AaRSs catalyze the attachment of the correct amino acid to its cognate tRNA which then is used in protein synthesis on ribosomes. Phylogenetically phenylalanyl-tRNA synthetase (PheRS), belongs to the class II aaRSs, and it is a dimer of heterodimers (αβ)2, containing two α- (PheS) and two β- (PheT) subunits. Structural studies of PheRS have shown that the α subunit binds L-Phe and ATP and is responsible for esterification catalysis. At the same time, the β subunit is involved in the recognition of the cognate tRNA molecule and editing of mis-charged tRNA.

The protein-fragment interactions were analyzed using crystal structures for five of those fragments complexed with MtPheRS/tRNAPhe (DDD00107555 (D-555), DDD01008876 (D-876), DDD00805735 (D-735), DDD00079004 (D-004) and DDD00067116 (D-116)). The FMO analysis indicates that the sulphonamide group of the D-735 interacts with αArg201 and αGln158 through strong hydrogen bonds. Also, the aniline nitrogen form hydrogen bond with the αGlu217 of D-735 fragment. Synthesis of L-Phe-AMP was inhibited the least by D-735 fragment. In the present study, the 3’ CCA tail of the tRNAPhe in the αβ heterodimer bound to D-735 was translocated into the editing domain, revealing the tRNA conformation during post-transfer editing. In one of the αβ heterodimer of the MtPheRS/tRNAPhe (αβ)2 complex bound to D-735, clear electron density directed towards the β3 and β4 domains of the β subunit was observed. We modeled the 3′ CCA end of the tRNAPhe acceptor stem into this density. An electron density that may be unambiguously attributed to the terminal A76 of the tRNAPhe was present in the deep, narrow tunnel that forms at the interface between the β3 and β4 domains of the β subunit. The D-735 compound occupying the synthetic site is separated by ~36 Å from acceptor end of tRNAPhe within the editing site. Our structural data of one of the αβ heterodimer of MtPheRS/tRNAPhe bound to D-735 provides the experimental validation of the water-mediated hydrolytic mechanism of ester cleavage in the editing site.

>[2x]AMLSPEALTTAVDAAQQAIALADTLDVLARVKTEHLGDRSPLALARQALAVLPKEQRAEAGKRVNAARNAAQRSYDERLATLRAERDAAVLVAEGIDVTLPSTRVPAGARHPIIMLAEHVADTFIAMGWELAEGPEVETEQFNFDALNFPADHPARGEQDTFYIAPEDSRQLLRTHTSPVQIRTLLARELPVYIISIGRTFRTDELDATHTPIFHQVEGLAVDRGLSMAHLRGTLDAFARAEFGPSARTRIRPHFFPFTEPSAEVDVWFANKIGGAAWVEWGGCGMVHPNVLRATGIDPDLYSGFAFGMGLERTLQFRNGIPDMRDMVEGDVRFSLPFGVGA;>[2x]QSNAMRLPYSWLREVVAVGASGWDVTPGELEQTLLRIGHEVEEVIPLGPVDGPVTVGRVADIEELTGYKKPIRACAVDIGDRQYREIICGATNFAVGDLVVVALPGATLPGGFTISARKAYGRNSDGMICSAAELNLGADHSGILVLPPGAAEPGADGAGVLGLDDVVFHLAITPDRGYCMSVRGLARELACAYDLDFVDPASNSRVPPLPIEGPAWPLTVQPETGVRRFALRPVIGIDPAAVSPWWLQRRLLLCGIRATCPAVDVTNYVMLELGHPMHAHDRNRISGTLGVRFARSGETAVTLDGIERKLDTADVLIVDDAATAAIGGVMGAASTEVRADSTDVLLEAAIWDPAAVSRTQRRLHLPSEAARRYERTVDPAISVAALDRCARLLADIAGGEVSPTLTDWRGDPPCDDWSPPPIRMGVDVPDRIAGVAYPQGTTARRLAQIGAVVTHDGDTLTVTPPSWRPDLRQPADLVEEVLRLEGLEVIPSVLPPAPAGRGLTAGQQRRRTIGRSLALSGYVEILPTPFLPAGVFDLWGLEADDSRRMTTRVLNPLEADRPQLATTLLPALLEALVRNVSRGLVDVALFAIAQVVQPTEQTRGVGLIPVDRRPTDDEIAMLDASLPRQPQHVAAVLAGLREPRGPWGPGRPVEAADAFEAVRIIARASRVDVTLRPAQYLPWHPGRCAQVFVGESSVGHAGQLHPAVIERSGLPKGTCAVELNLDAIPCSAPLPAPRVSPYPAVFQDVSLVVAADIPAQAVADAVRAGAGDLLEDIALFDVFTGPQIGEHRKSLTFALRFRAPDRTLTEDDASAARDAAVQSAAERVGAVLRG> DQAGKSPNAVRYHGGDEIILQGFHWNVVREAPNDWYNILRQQAATIAADGFSAIWMPVPWR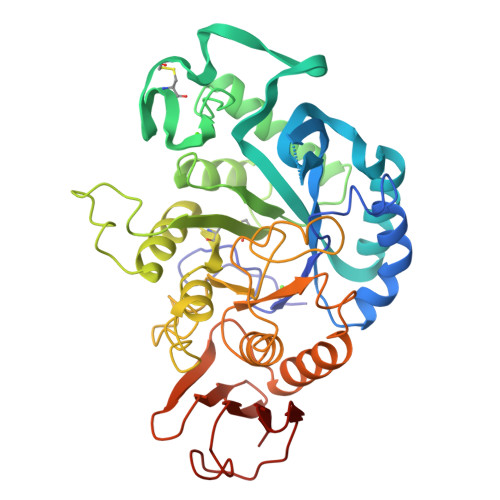DFSSWSDGSKSGGGEGYFWHDFNKNGRYGSDAQLRQAASALGGAGVKVLYDVVPNHMNRGYPDKEINLPAGQGFWRNDCADPGNYPNDCDDGDRFIGGDADLNTGHPQVYGMFRDEFTNLRSQYGAGGFRFDFVRGYAPERVNSWMTDSADNSFCVGELWKGPSEYPNWDWRNTASWQQIIKDWSDRAKCPVFDFALKERMQNGSIADWKHGLNGNPDPRWREVAVTFVDNHDTGYSPGQNGGQHHWALQDGLIRQAYAYILTSPGTPVVYWDHMYDWGYGDFIRQLIQVRRAAGVRADSAISFHSGYSGLVATVSGSQQTLVVALNSDLGNPGQVASGSFSEAVNASNGQVRVWRS> GSHMASMTGGQQMGRGSEFARENEMDENLEQVSGIIGNLRHMALDMGNEIDTQNRQIDRIMEKA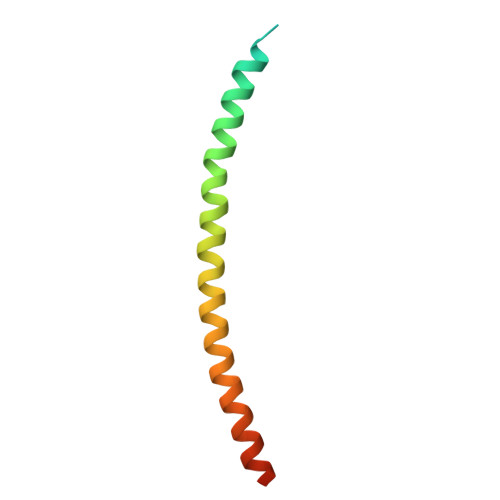DSNKTRIDEANQRATKML> MAMPDVQYPINTYGWLKKAVALWADRDDDEFVNQIPNFINFAEKEIYRNLRIPPLEKEVYLDIKDGVAYIPPDYLEAQWMMRAKDGTIFQVTSPEEISYRRQHGTINPSHWNNQPVNFARFGSRFIFYPSIEADTPYYPDDGSPLIPAENSVILSYYADPPEFHEDTDTSTILTIAPELLLYFTLRHACLFVQDDNGVQKWSALGKAILDEMVEQNKKQEYSGSPI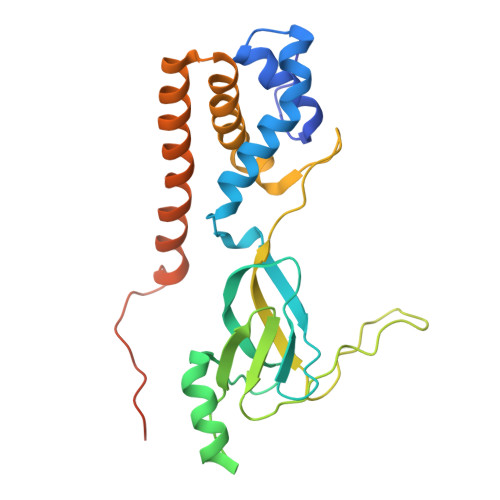AIPNNMTRLQSSLPDIYGIRTSRV> RNDYVQEEKQQQLQEPLDGQWKPTTTGHDAIVPFSEPKPVTISEKAGVKFKPLLDVNTGCAPYAAVNAEGETSGGLQTSGDPESGCRGSKYGSQVYGRSTWYNDVWAIMYAWYFPKDSPMLLMGHRHDWENVVVFINDPDEVEPTILGCSTSWHSGYIKYAPCPTDSINGSSVMIKYEHSFPLNHALNITKDAGAYQDLIMWHQMPDLARRALNDTDFGKAITPMNDLNFMEKIE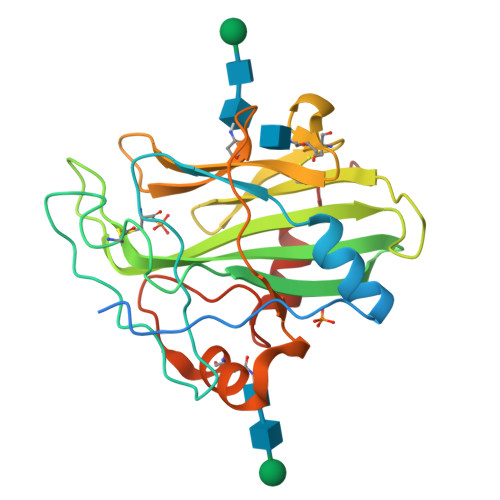AAWPFKTKKDGA>[24x]MLSRSRCVSRAFSRSLSAFQKGNCPLGRRSLPGISLCQGPGYPDSRKIVISNSSVLNVRFFRTTAVCKDDVITVKTPAFAESVTEGDVRWEKAVGDTVAEDEVVCEIETDKTSVQVPSPANGVIEALLVPDGGKVEGGTPLFTLRKTGAAPAKAKPAEAPAAAAPKAEPAVSAVPPPPAASIPTQMPPVPSPPQPLTSKPVSAVKPTAAPPVAEPGAVKGLRAEHREKMNRMRQRIAQRLKEA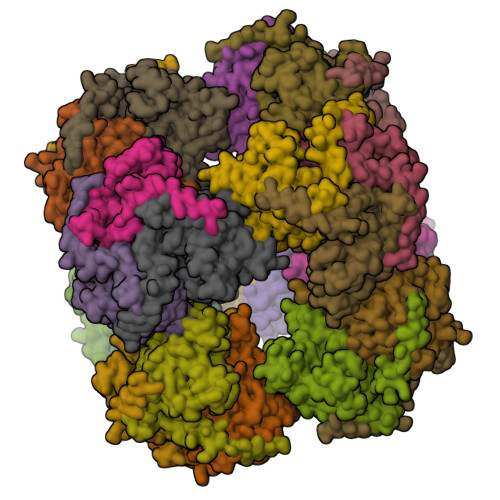QNTCAMLTTFNEIDMSNIQDMRARHKEAFLKKHNLKLGFMSAFVKASAFALQEQPVVNAVIDDTTKEVVYRDYIDISVAVATPRGLVVPVIRNVETMNYADIERTISELGEKARKNELAIEDMDGGTFTISNGGVFGSLFGTPIINPPQSAILGMHAIVDRPVAVGGKVEIRPMMYVALTYDHRLIDGREAVTFLRKIKAAVEDPRVLLLDL>SRGTAGAPMRGYKVTDNERTRKYGIGANSLEMLIAKAKSKFPLLEPHLYLASDGFEVSDDEYLKSLPAQTLFIVSGPDAVITTDADFEFEKMLEHHHHH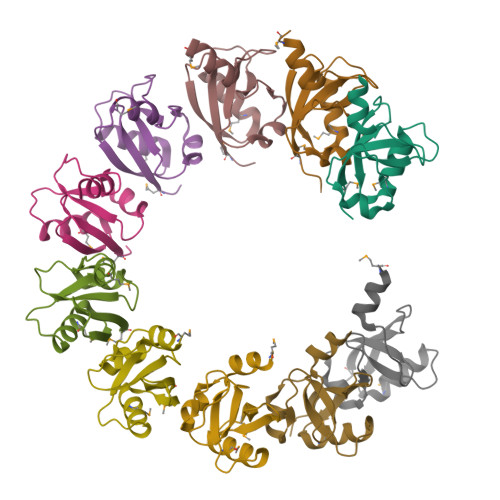H[10x]> GHAIHDSAINYLVLLDQLEWQRSDNTNNFSWSVNSWIGGDTDRIWLKSEG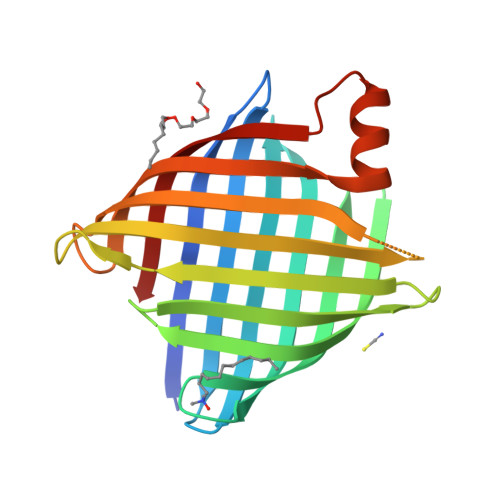ERSNGETEAAEAQLLWGHAVGPWWDLVAGVRQDFRPASARTWAAVGFQGLALYNFESEITGFVSNGGKAALRLGGEYDVLLTNRLILQPSYEVNFYSQDDESRGRGRGLTDTELGLRLRYEIRREFAPYIGVSWNQLYGKTSDMAKREGEKDHQVVFLAGARIWF> SVGTSCIPGMAIPHNPLDSCRWYVSTRTCGVGPRLATQEMKARCCRQLEAIPAYCRCEAVRILMDGVVTSSGQHEGRLLQDL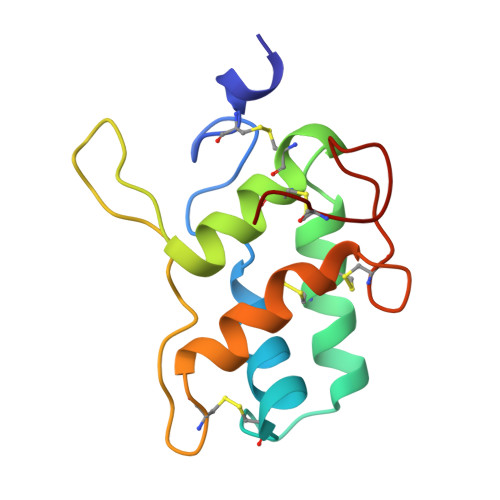PGCPRQVQRAFAPKLVTEVECNLATIHGGPFCLSL Here, we characterize the structure and function of a thermophilic dNDT, the protein from Chroococcidiopsis thermalis (CtNDT). Nucleoside 2′-deoxyribosyltransferase (dNDT) enzymes catalyze transglycosylation via a covalent 2′-deoxyribosylated enzyme intermediate with retention of configuration, having applications in the biocatalytic synthesis of 2′-deoxynucleoside analogues in a single step. The reaction catalyzed by dNDT proceeds via a ping-pong mechanism, with the formation of a 2′-deoxyribosyl-enzyme intermediate covalently linked to an active-site glutamate.13 Transglycosylation occurs in a stereospecific manner, preserving the anomeric carbon in the β configuration in the newly formed 2′-deoxyribonucleoside. As with other NDT enzymes, the active site of CtNDT is formed by residues from two monomers, and therefore, it is only fully formed in the dimer/tetramer.

Prior work with the LhNDT13 trapped a 2′-deoxy-2′-fluoro-ribosyl intermediate upon incubation with a 2′-deoxy-2′-fluoro-β-d-arabinofuranosyladenine substrate, and it was hypothesized that 2′-fluoro-containing substrates undergo slower hydrolysis in comparison to compounds lacking fluorine on position 2′. We report a structure of a 2-difluoro-2-deoxy-ribosylated CtNDT after cocrystallization with Gemcitabine for comparison with the ribosylated enzyme. Figure S17 shows a comparison between ribosylated and 2-difluoro-2-deoxy-ribosylated CtNDT. The main difference is in the conformation sampled by the 3′-OH of the 2-difluoro-2-deoxy-ribosylated intermediate, positioned closer to S10 than to D62. After the ligand was added to the protein, refinement (with Phenix Refine) produced three monomers with a covalently modified E88 and one with a covalent modification on D62. We do not have additional biochemical evidence for the formation of a covalent intermediate with D62, and because this could be an artifact, we have not discussed this in detail.

>[4x]GMKRKIIYLASPYGFSQQQKTLLLPPIVRALEALGIEVWEPFARNNQIDFSQADWAYRVAQADLQDVKNCDGIFAVVNGTPPDEGVMVELGMAIALNKAIFLFRDDFRRCSDNERYPLNLMLFAGLPEIGWENYYYTSVDEIQSHDKALYKWLTGM> MSPILGYWKIKGLVQPTRLLLEYLEEKYEEHLYERDEGDKWRNKKFELGLEFPNLPYYIDGDVKLTQSMAIIRYIADKHNMLGGCPKERAEISMLEGAVLDIRYGVSRIAYSKDFETLKVDFLSKLPEMLKMFEDRLCHKTYLNGDHVTHPDFMLYDALDVVLYMDPMCLDAFPKLVCFKKRIEAIPQIDKYLKSSKYIAWPLQGWQATFGGGDHPPKSDLVPRGSPEFMADGVRAVVADDSHFMRSVISDILSDGGIDVVAQARDGEEAVSAVIEHRPDVVTMDVEMPVMNGIEATERIMAESPTPVLMLSAHTDENADVTFEALDKGAVDFFTKPGGEVSMEMSRLKDQLVEMVSSVAAVDVGATGSRSGTGSDSGTAPTTAGGSATDRRGTGGSSGQTTYVANPTLVIGSSTGGPKMVEQVMENLPIEADLRVLIIQHMPEGFTGRFAERINTRSDYEVQEATDGARIGGGEGLVAAGDRHMEVKNYRNGRLRTKLTQDEPVNSVRPAVDVTMQTAAET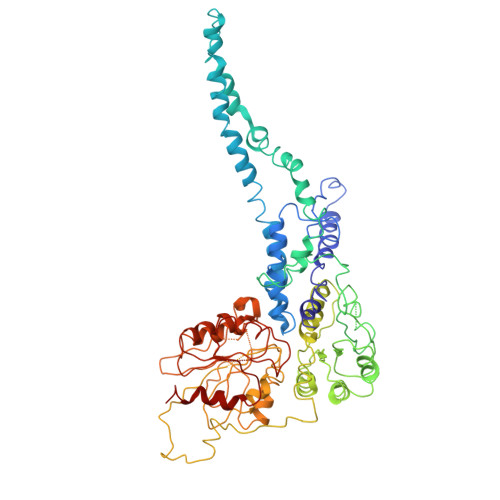IDDPLVGLILTGMGEDGADGIRRIKQAGGKTIAQDEATSAVYGMPKRAAETGCVDTVLPIDDIADGVIDTITTEVT> TLWDTTVRLSETMTLECVYPLTHNLTQVEWTKNTGTKTVSIAVYNPNHNMHIESNYLH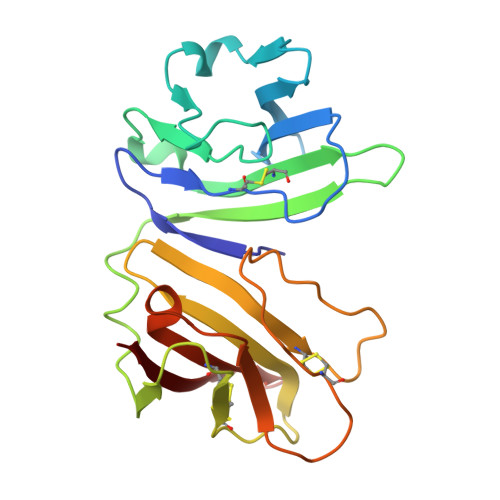RVHFLNSTVGFRNMSLSFYNASEADIGIYSCLFHAFPNGPWEKKIKVVWSDSFEIAAPSDSYLSAEPGQDVTLTCQLPRTWPVQQVIWEKVQPHQVDILASCNLSQETRYTSKYLRQTRSNCSQGSMKSILIIPNAMAADSGLYRCRSEAITGKNKSFVIRLIIT>[6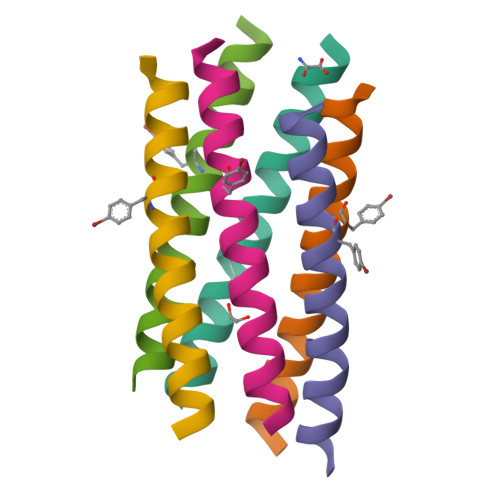x]XGEFAQAVKEYAKAVKEYAYAVKEFAQAVKGX> GCRLRSQL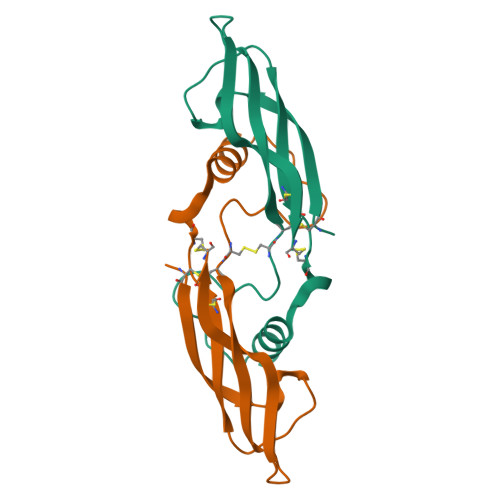VPVRALGLGHRSDELVRFRFCSGSCRRARSPHDLSLASLLGAGALRPPPGSRPVSQPCCRPTRYEAVSFMDVNSTWRTVDRLSATACGCLGHHHHHH> SLMLLSPAQVAGSWTFYVQGAEQDACTVTLKKDRTFSAQVSCLQAWLGRTPTTWS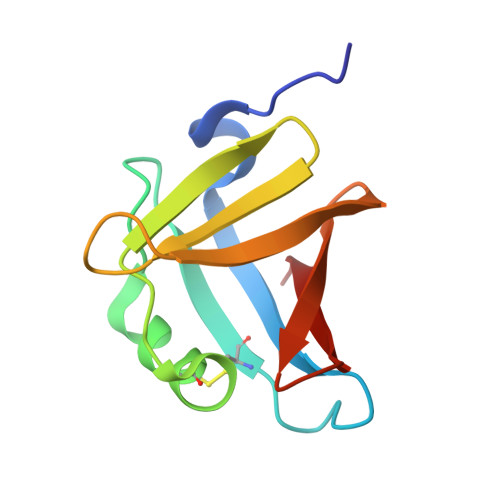PTPDGLLLIGKDGSQSLFLELREAGRYEGSVEGSKTLVMQRA2,5-DIPHENYLFURAN-3,4-DICARBOXYLIC ACID | C18 H12 O5 | 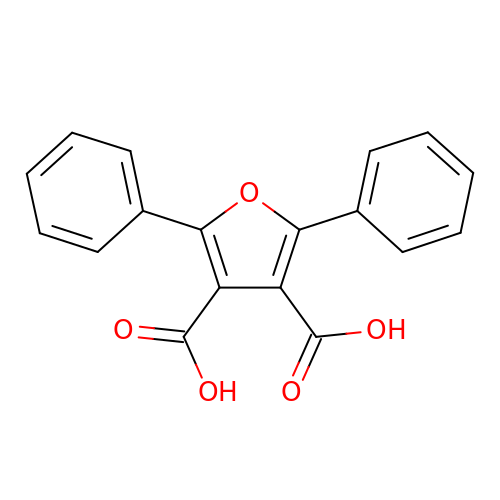QPKYPOMZPFDBEZ-UHFFFAOYSA-N> NECIVETRTTRISGRDA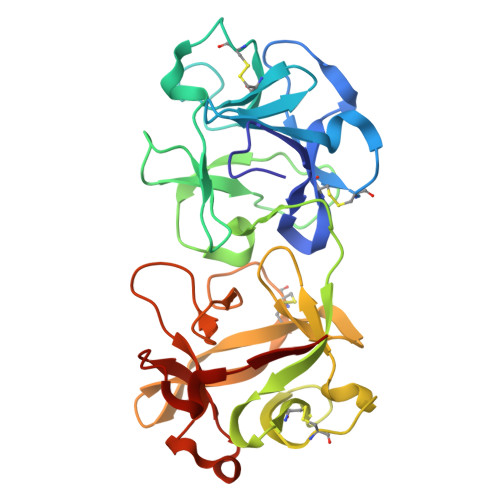LCVDVAGALTSDGSRLILYPCGQQVNQKWTFHSDGTVRSLGKCLATNNSKFGNLVVIYDCSKLAAEDISWDVSVGGTIMNPNYEDLALTSNKATRSTNLTMEVNTYSASQGWRVGNYVQPIIGSIVGLDDMCLEATDGNTNMWLEECVPNKREQSWALYSDGTIRVDDNRELCVTASSSTYDNWKVITILNCDGSNNQRWVFLADGSISTPGNQRLAMDVARSDVDLKKIILHRPHGDLNQQWVLFY> GINPPSGVTEKQLSDDELMTLVQKQTFRYFWDFAHPESGLAHERSNGGAETATIGGSGFGVMAIIVGIERGFVTREQGAERMLKIVRFLSDKNTDSYHGMWAHWMNGKTGKTIPFSRKDDGADIVESAFMFEGLLAAHQYFTKDNPTENRIRGIINNLWRQAEWNFFTQGQD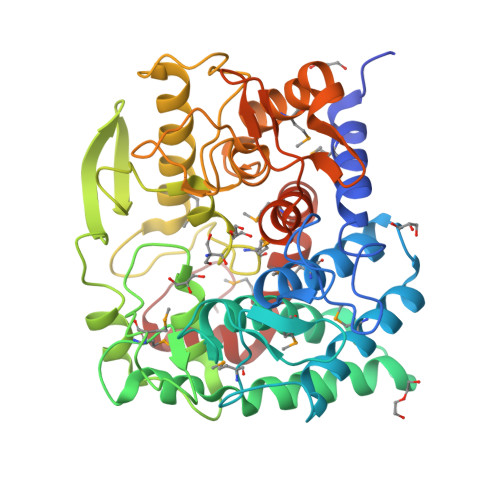VMYWHWSPNNGWAMNHQIKGHNECHIVYILGASSPTYPIAESVYHKGWANANTFLNGREYYGIKLPLGNNHGKGGPLFFTHYSYMGLDPRGLKDRYADYEEQMKAHTLINRAYCIDNPKGYKGYGEKCWGLTASDGDKGYSAHSPGNDRGVITPTAALSSIPYAPEYSLEAMRYFYEELGDRLWGEYGFKDAFNLTENWFAPSYLAIDQGPIIVMIENYRTGLIWKLFMSHPDVQKGLRRLGFTSPYLNKVD>MMSETAPLPSASSALEDKAASAPVVGIIMGSQSDWETMRHADALLTELEIPHETLIVSAHRTPDRLADYARTAAERGLNVIIAGAGGAANLPGMCAAWTRLPVLGVPVESRALKGMDSLLSIVQMP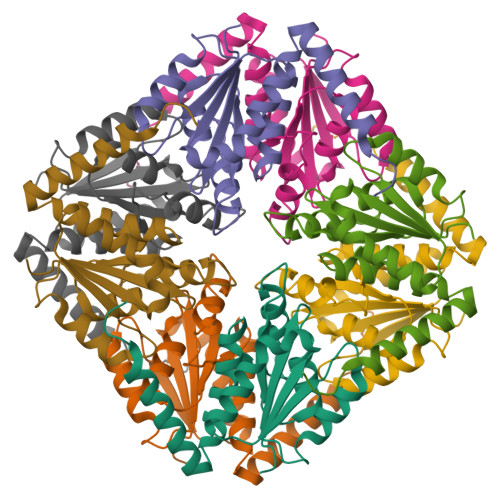GGVPVGTLAIGASGAKNAALLAASILALYNPALAARLETWRALQTASVPNSPITEDK[2x]> GSGTAAQPAPLTASMLASAPPQEQ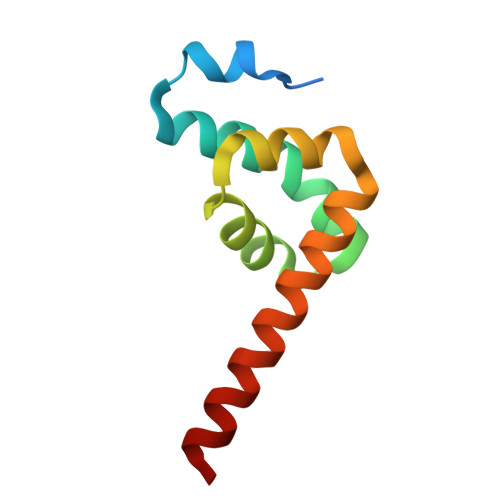KQMLGERLFPLIQAMHPTLAGKITGMLLEIDNSELLHMLESPESLRSKVDEAVAVLQAHQAKEAAAAA>[2x]GLETSSKKYSLGKTLGTGSFGIVCEVFDIESGKRFALKKVLQDPRYKNRELDIMKVLDHVNIIKLVDYFYTTGDEEPKPPQPPDDHNKLGGKNNGVNNHHKSVIVNPSQNKYLNVIMEYVPDTLHKVLKSFIRSGRSIPMNLISIYIYQLFRAVGFIHSLGICHRDIKP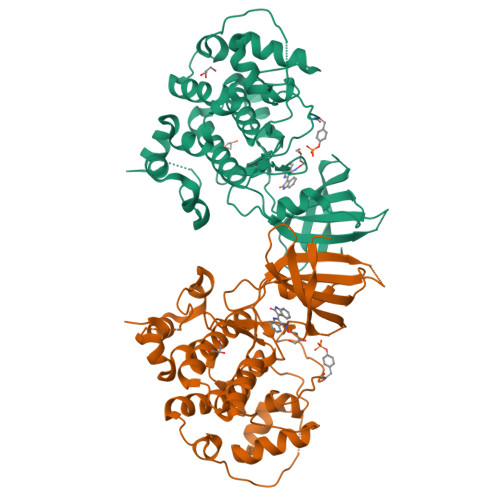QNLLVNSKDNTLKLCDFGSAKKLIPSEPSVAYICSRFYRAPELMLGATEYTPSIDLWSIGCVFGELILGKPLFSGETSIDQLVRIIQIMGTPTKEQMIRMNPHYTEVRFPTLKAKDWRKILPEGTPSLAIDLLEQILRYEPDLRINPYEAMAHPFFDHLRNSYESEVKNNSNFPHGVNQNIPQLFNFSPYELSIIPGNVLNRILPKNFSPNYKH GENETICIN | C20 H40 N4 O10 | 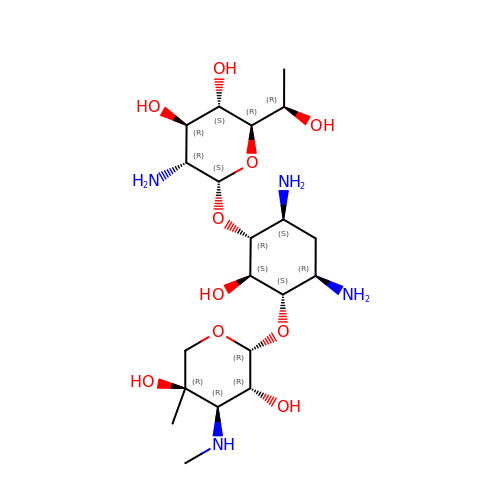BRZYSWJRSDMWLG-DJWUNRQOSA-N>MIKNIITTIDDYARTQPNNVVYDVQGVTHTYAELKAYSDALAAHLDTLDLPAKDPIIVFGGQTFEMIATFLGVVKSGRAYIPIDTHSPNERLTMINEIAKPAAVIAVADLPTGVGTTPVITPDQLAAIFATPVDYQADHVVSGDDNYYIIFTSGTTGMPKGVQISHDNLVSYVDWMLSDDFGLPDQPNSLSQPPYSFDLSVMDVYPTLALGGTLYALPKAVTDDFKQLFAALPTLPINVWVSTPSFMDICLLEPKFNAENLPTLTHFLFCGEELTHKTAATLKKRFPDARIFNTYGPTETCVAVTQIEITDAALAQYDRLPIGYAKADTRILVVDENGEAVPNGTEGELIIAGPSVSKGYLNNPEKTAKAFFELDGQPAYHSGDIGTMDADGLFRYRGRVDFQIKMHGYRIELEEVDHFLAQQQHIKQAVAVPKYDKEHKVTQMIAYVVPKPNDFESDFALTTAIKKDLQGMMMEYMIPQRFVYQTSLPLTPNGKIDVKSIIKEVNPE[2x]

TA d-alanylation is performed by the Dlt pathway, which starts in the cytoplasm and continues extracellularly after d-Ala transportation through the membrane. The first step in the d-alanylation mechanism of TA is the transfer of the phosphopantetheinyl moiety of coenzyme A (Ppant) to the DltC protein by the Phosphopantetheinyl transferase AcpS. The d-alanine-d-alanyl carrier protein ligase (DltA) catalyzes a two-step reaction: the activation of d-Ala using ATP to form a d-alanyl-AMP intermediate and then the transfer of d-Ala as a thiol ester to the Ppant group of DltC. Altogether, we conclude that DltC1 acts as an interaction hub for all the successive cytoplasmic steps of the TA d-alanylation pathway.

To investigate this mechanism, we produced and purified L. plantarum DltA and solved its crystal structure at 2.1 Å resolution. The asymmetric unit of the crystal contains two DltA molecules which are largely similar (rmsd of 0.5 Å on 392 residues). The last 100 aminoacids constituting the C-terminal minor domain are not visible in the electron density although present in the purified sample. The overall structure of the large N-terminal domain (residues 3–395) is composed of three subdomains (referred in previous studies as subdomains A, B and C39) two of which, A and B, sharing a similar topology with a β-sheet flanked on both sides by α -helices. As crystallization was achieved in the presence of d-Ala and ATP, one molecule of d-Ala-AMP could be observed in the electron density of one DltA molecule of the asymmetric unit. The d-Ala-AMP binding cleft of DltA is defined at the interface between loop 270–274, the β strands β13 (residues 290–295), β14 (residues 305–308) and β21 (residues 394–399) and the P-loop (phosphate binding loop or Walker A motif) comprised between residues 152 and 160. More precisely, the adenine ring is sandwiched between residues Gly271 and Glu272 on one side and Tyr295 on the other side. In our DltA structure, the P-loop is well defined in one molecule of the asymmetric unit. Although no direct interaction is established with the d-Ala-AMP, a locally positively charged environment mainly through the Lys160 is created in the vicinity of the phosphate group. These new structural data suggest that the P-loop could therefore contribute to the stabilization of the substrate binding.> KLHIPVMVDEVVHCLSPQKGQIFLDMTFGSGGHTKAILQKESDIVLYALDRDPTAYALAEHLSELYPKQIRAMLGQFSQAEALLMKAGVQPGTFDGVLMDLGCSSMQLDTPERGFSLRKDGPLDMRMDGGRYPDMPTAADVVNALDQQALASILRTYGEEKHA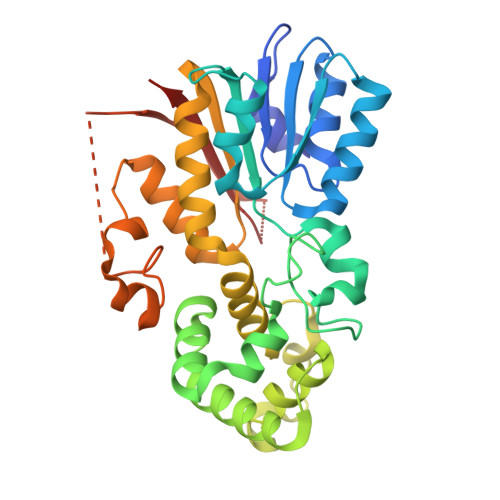KKIASAIVQARSIYPITRTQQLASIVAGAFPPSAIYTRKDLLQRSTHIATKTFQALRIFVNNELNELYTGLKTAQKFLRPGGRLVALSFHSLEDRIVKRFLLGISMTERFNLSVRQQVMKTSQLGSDHENTEEVSMRRAPLMWELIHKKVLSPQDQDVQDNPRGRSAKLRAAIKL>[4x]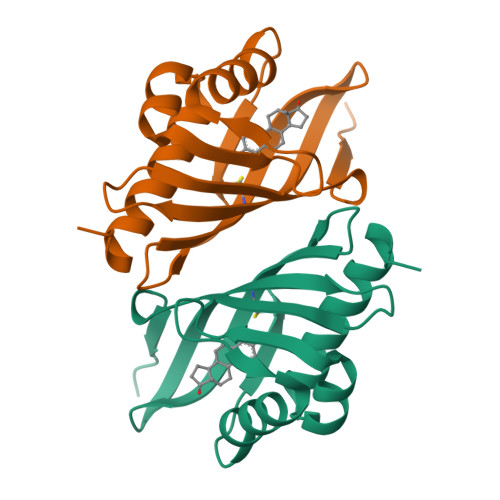MNLPTAQEVQGLMARYIELVDVGDIEAIVQMYADDATVENPFGQPPIHGREQIAAFYRQGLGGGKVRASLTGPVRASHNGSGAMPCRVEMVWNGQPSALDVIDVMRFDEHGRIQTMQAYWSEVNLSVREPQ>[4x]QRAGNETPENHPPLTWQRCTAPGNCQTVNAEVVIDANWRWLHDDNMQNCYDGNQWTNACSTATDCAEKCMIEGAGDYLGTYGASTSGDALTLKFVTKHEYGTNVGSRFYLMNGPDKYQMFNLMGNELAFDVDLSTVECGINSALYFVAMEEDGGMASYPSNQAGARYGTGYCDAQCARDLKFVGGKANIEGWKSSTSDPNAGVGPYGSCCAEIDVWESNAYAFAFTPHACTTNEYHV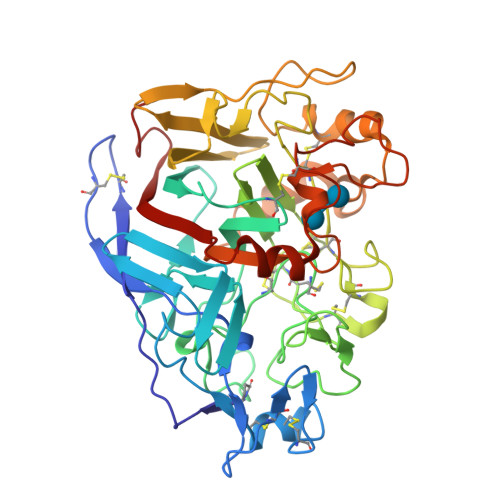CETTNCGGTYSEDRFAGKCDANGCDYNPYRMGNPDFYGKGKTLDTSRKFTVVSRFEENKLSQYFIQDGRKIEIPPPTWEGMPNSSEITPELCSTMFDVFNDRNRFEEVGGFEQLNNALRVPMVLVMSIWDDHYANMLWLDSIYPPEKEGQPGAARGDCPTDSGVPAEVEAQFPDAQVVWSNIRFGPIGSTYDF> GIDPFTARPSSSMADFRKFFAKAKHIVIISGAGVSAESGVPTFRGAGGYWRKWQAQDLATPLAFAHNPSRVWEFYHYRREVMGSKEPNAGHRAIAECETRLGKQGRRVVVITQNIDELHRKAGTKNLLEIHGSLFKTRCTSCGVVAENYKSPICPALS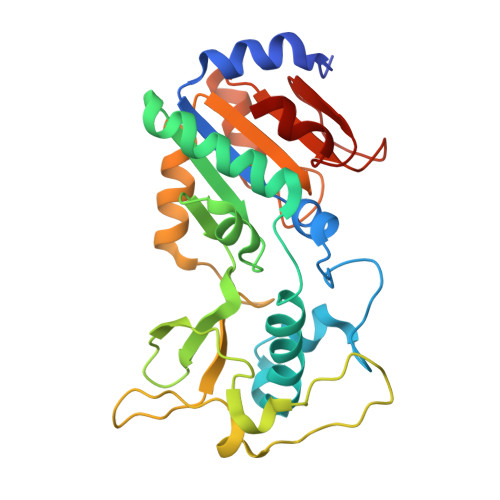GKGAPEPGTQDASIPVEKLPRCEEAGCGGLLRPHVVWFGENLDPAILEEVDRELAHCDLCLVVGTSSVVYPAAMFAPQVAARGVPVAEFNTETTPATNRFRFHFQGPCGTTLPEALA> IHEGPYPEPLVNLLDVVYYGPISIGTPPQDFQVIFDTGSANLWLPSSKCTTKYCLHHHR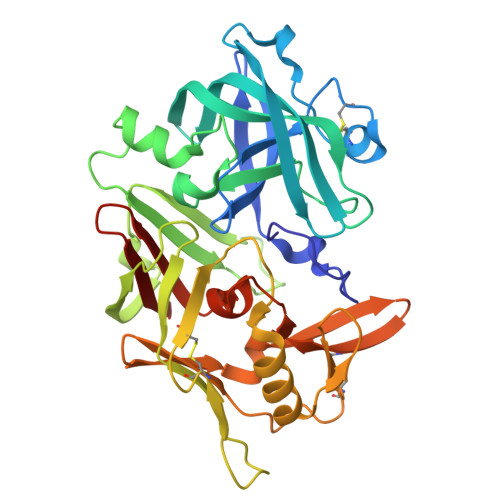YDSSKSSTYEADGRNFTIVYGSGNVEGFISKDVCRIGSAKVSGQPLGEALVVGGESLLEAPFDGILGLAYPSIAVDGVVPVFDNMMKQGLLGEQNVFSVYLNRDPSSKEGGEVLFGGIDHDHYKGSITYVPVTAKGYWQFHVDGVKSVSASKSAPELLCKDGCEAIANTGTSLITGPPEEVDSLNQYLGGTKTEGGQYLLDCDKLESLPNVTFTISGKEFSLRSKDYVLKVNQQGQTLCVSGFMGLEMPQPLWILGDVFLGPYYTIFDRDQDRVGFAEVAHHHHHH;> AFRIPLTR>RGSHHHHHHGSFTPSGTTGTTKLTVTEKCQVRVGDLTVAKTRGQLTDAAPIGPVTVQALGCDARQVALKADTDNFEQGKFFLISDNNRDKLYVNIRPTDNSAWTTDNGVFYKNDVGSWGGIIGIYVDGQQTNTPPGNYTLTLTGGYWAK[6x]

Dr adhesins are expressed on the surface of uropathogenic and diffusely adherent strains of Escherichia coli. The major adhesin subunit (DraE/AfaE) of these organelles mediates attachment of the bacterium to the surface of the host cell and possibly intracellular invasion through its recognition of the complement regulator decay-accelerating factor (DAF) and/or members of the carcinoembryonic antigen (CEA) family. The adhesin subunit of the Dr haemagglutinin, a Dr-family member, additionally binds type IV collagen and is inhibited in all its receptor interactions by the antibiotic chloram­phenicol (CLM). In this study, previous structural work is built upon by reporting the X-ray structures of DraE bound to two chloramphenicol derivatives: chloramphenicol succinate (CLS) and bromamphenicol (BRM).

Preparation of THM–DraE cocrystals was attempted in order to determine whether para substitutions of the nitro group affected the interaction with DraE. The aromatic ‘head’ group of THM comprises a para-substituted methyl phenyl sulfone moiety. Soaks of THM into CLS cocrystals were attempted based on the assumption that the tetrahedral methyl sulfone group of THM could be distinguished from the planar nitro group of CLS in the electron density. Indeed, CLS refined successfully at full occupancy and no residual peaks were observed in the difference map. Therefore, we concluded that THM was unable to enter the CLM-binding pocket of DraE in the P3 crystal form. Steric interference between the protein and the methylsulfonyl group of THM is the most likely reason for this. THM occupied the same nonphysiological binding site as BRM. The entire THM molecule was traced within this difference density and no negative peaks were observed in the difference map after refinement with 100% THM occupancy. The two THM molecules in the ASU adopt a similar conformation to CLM in the physio­logical binding site and are positioned at the interface between two subunit copies. In more detail, hydrogen bonds are formed between the carbonyl of THM and the main-chain amide of Val105, the primary hydroxyl group OH(3) of THM forms hydrogen bonds to the side-chain atoms of Asp104 on one subunit (chains F and C) and Thr36 on the other (chains D and B), and a hydrogen bond occurs between the main-chain carbonyl of Gly33 and the amide within the aliphatic tail of THM.> MRGSHHHHHHGSENLYFQATTTLNDSVTTTLASEPQRTYQVVVAATKEMGIGKDGKLPWNLPTDLKFFKDITLTTSDSSKKNAVVMGRKTWESIPIKYRPLSGRLNVVLTRSGGFDIANTENVVTCSSVDSALDLLAAPPYCLSIERVFVIGGGDILREALNRPSCDAIHLTEIDTSVDCDTFIPAIDTSVYQPWSSSFPVTENGLRFCFTTFVRVKSSADESSDESNGSQSLQFDGKKFLFLPKMVFDQHEEFLYLNMVEDIISNGNVKNDRTGTGTLSKFGCQMKFNLRRSFPLLTTKRVFWRGVVEELLWFISGS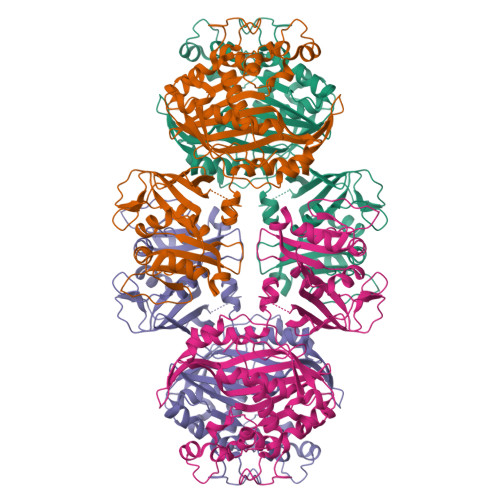TNAKVLQEKGIHIWDGNASREYLDGIGLTEREEGDLGPVYGFQWRHFGAKYTDMHADYTGQGFDQLVDVIDKIKNNPDDRRIIMSAWNPSDLKLMALPPCHMFAQFYVAEGELSCQMYQRSADMGLGVPFNIASYSLLTCMLAHVCDLVPGDFIHVLGDAHVYKTHVRPLQEQLLNLPKPFPVMKINPEKKQIDSFVASDFDLTGYDPHKKIEMKMAV> KLS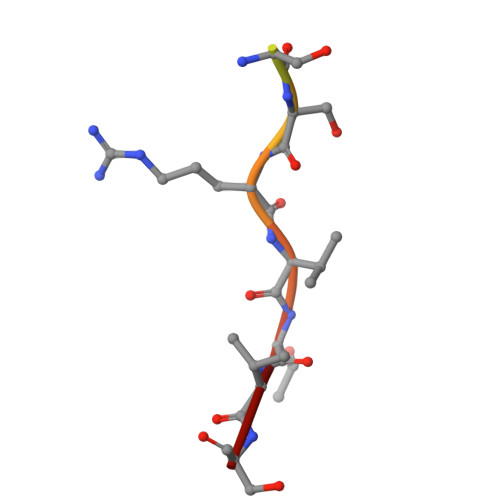PSPSSRVTVS Here, we show that a tyrosine phosphoregulatory system controls the biosynthesis and abundance of Vibrio exopolysaccharide (VPS), an essential biofilm component of the pathogen Vibrio cholerae. The phosphorylation state of the tyrosine autokinase VpsO, mediated by the tyrosine phosphatase VpsU, directly modulates VPS production and also affects the kinase’s own degradation, to regulate VPS production. We found that VpsO and VpsU have respective kinase and phosphatase functions, and we have determined crystal structures of VpsU and the VpsO catalytic domain. We found that the VpsU tyrosine phosphatase controls VPS production through regulation of the VpsO phosphorylation state. Together, our data suggest that the phosphorylation state of the C-terminal tail of VpsO, modulated by autokinase and VpsU phosphatase activity, regulates the functional state of VpsO to control VPS production and biofilm formation in V. cholerae.

We found that the only version of VpsO-503 that we could crystallize was VpsO-503E519A, R522A, R525A, which contains mutations in a conserved ExxRxxR motif in the kinase domain (E519, R522, R525). We determined the structure of VpsO-503E519A, R522A, R525A from x-ray diffraction data at a resolution of 2.9 Å. Two VpsO molecules are present in the asymmetric unit; these molecules dimerize through the α1 helix, which contains the mutated ExxRxxR motif. The kinase domain adopts the expected α/β mononucleotide-binding fold with a seven-stranded β-sheet surrounded by eight α-helices. In contrast, the VpsO-503E519A, R522A, R525A protein used for crystallization lacks the N-terminal extension found in other BY-kinases, and alternatively, its α1 helix is longer at its N-terminus. This helix likely contacts the adenine base of ATP, and it contains two glutamates (E512 and E516) that could coordinate the ribose. Refinement of the VpsO structure revealed unmodeled electron density in the ATP binding site that is consistent with the presence of a phosphorylated tyrosine residue. The phosphate is located in a position similar to that of the β-phosphate of ADP in the Wzc structure. It is coordinated through hydrogen bonding to backbone amides (residues 548–550) in the P-loop and through T552, which are all part of the canonical Walker A motif. In addition, R583 stacks against the tyrosine aromatic ring. The position of the phosphotyrosine suggests that it should inhibit nucleotide binding, and we do not observe ADP in the active site despite its presence at 1 mM in the crystallization buffer.

>KLDAKAYFDEKLRELTAAVATIATSYLLAHVNQDQHVVMLTSCLPGEGKTTSSLNLALSLAQMEKTLLIDCDLRKPAIAHRFGISGSQPGVTNLLNGTQSLEDCVYHDEQSGLDILTAGVYASNPLELLSSSKFSELLADLRTRYQRIVIDTPPCLAVSDSFMLAQYVDSVILVIDANHTRTPVVREVVGKLTQQGSRIDGVILNRLNAKKASRYSGYYHYQAYYGEETKSGAAK[2x]> TPFIRPDMKAFLEAIAAMAGPTLAEMTLEEARASYVALHGMADRPARELAVIRNLSCPGPAGDIPLRLYDARESREAGPVITFYHGGGFVIGDLDTHHNLCTEIAALMDLPVVAVDYRLAPEHP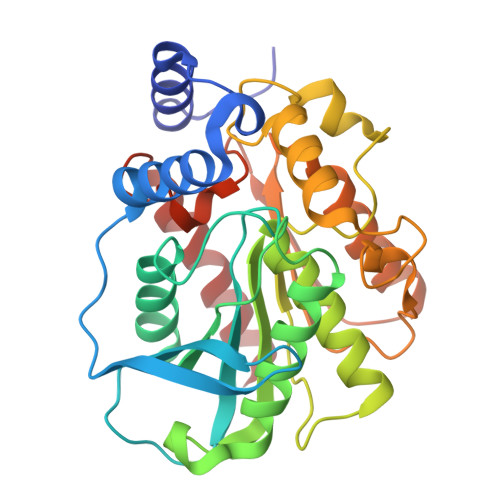FPAAIEDCEAATRWVASSPSELGRTASGVIPIGDAAGGNATIVVSQLLGAKPADVPVVLQVPIFPLASDAVGSASLEAFAEGFVLTKASIEFFDTAYKADRADPRGFPILGDHTAAPPTIVATASLDPIRDSGRDYAKALVEAGRDVVYLEMEGVTHSFTNIRAAVPSTQGDLERIIAAMKMMLG C-di-GMP is a near-ubiquitous bacterial second messenger responsible for the coordination of a variety of cellular processes and behaviour, including motility, biofilm formation, virulence and cell cycle progression. DGCs catalyse the condensation of two molecules of GTP to yield the twofold symmetric c-di-GMP product. DgcR from Leptospira biflexa is a constitutively dimeric prototype of this class of diguanylate cyclases. Here, we show by biophysical and crystallographic analyses that DgcR is a constitutive dimer that changes coiled-coil geometry and domain arrangement upon pseudo-phosphorylation.

A DgcR variant (R206A/D209A, abbreviated DgcR_AxxA) that had the putative allosteric inhibition site mutated was used to avoid locking the enzyme in a product-inhibited conformation. Crystallisation was performed in presence of 3’-deoxy-GTP (3’dGTP), which is a non-competent substrate analogue due to the absence of the 3’-hydroxyl group. The structure of native DgcR_AxxA (called DgcR’) was solved by molecular replacement to 2.2 Å resolution. There is one dimer in the asymmetric unit with the protomers held together by extensive isologous contacts between the Rec domains involving their α4-β5-α5 face. Notably, the electron density of the Rec domains is considerably weaker than that of the GGDEF domains, indicating a larger mobility. The GGDEF domains do not obey the twofold symmetry of the Rec domains, but form a relative angle of about 90°. Thus, the two active sites with the bound GTP analogues do not face each other rendering this constellation clearly non-productive. Though the constellation may be determined to some extent by crystal packing, it demonstrates considerable inter-domain flexibility. Comparison of the main-chain torsion angles reveals that the relative rotation can be traced back to a 169° change in a single torsion, namely around the Cα–C bond of residue 136 (ψ136). The native Rec dimer with a buried surface area of 980 Å2 is held together by an extended apolar contact of α5 (A117, F120) with α4 (F94, I98), an ionic interaction of D104 with R118, an H-bond between main-chain carbonyl 102 and R124 (both β5-α5 contacts).

>[2x]RKILIIEDSELQRKLLSRWVSKNGYIAIEAESISVAREKIISESIDVVLLDWELPDGNGIDLISDILSTSPVGWLPIIMVTGHTEPEYFKIAIEAGATDYITKPAKEIELLARIFSALRIKALHDQLRETAIRDVMTGLYNRRYMEERIEQEFQRCKRHDSLLSMAMIDIDKFKNINDTYGHEIGDQVIKQLAHELKTSFAKSAIISRFGGEEFVILFPETGVVDATRILDRVRENVSKLEMKSDTDQIFHFTFSGGVAGGDLSDIQSNQELLKIADKNLYEAKSSGRNQIIS> LASNGDKIESFVPKEGKKTGNKF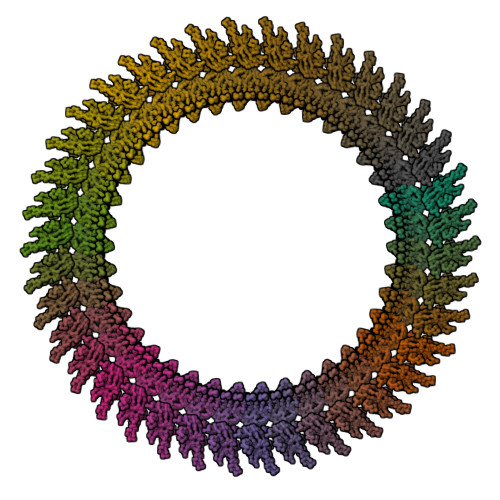IVVERQKRSLTTSPVDISIIDSVNDRTYPGALQLADKAFVENRPTILMVKRKPININIDLPGLKGENSIKVDDPTYGKVSGAIDELVSKWNEKYSSTHTLPARTQYSESMVYSKSQISSALNVNAKVLENSLGVDFNAVANNEKKVMILAYKQIFYTVSADLPKNPSDLFDDSVTFNDLKQKGVSNEAPPLMVSNVAYGRTIYVKLETTSSSKDVQAAFKALIKNTDIKNSQQYKDIYENSSFTAVVLGGDAQEHNKVVTKDFDEIRKVIKDNATFSTKNPAYPISYTSVFLKDNSVAAVHNKTDYIETTSTEYSKGKINLDHSGAYVAQFEVAWDEVSYDKEGNEVLTHKTWDGNYQDKTAHYSTVIPLEANARNIRIKARECTGLAWEWWRDVISEYDVPLTNNINVSIWGTTLYPGSSITYN> MNSLSSKKANSLVFKSIRNFTLQWGSLAERPMVDRVMSTSTWPVPYYQRLFKAYPIREKKDKMSLLLSDIDIDDTNWYQAKDFLRGSFRGRQIVDYVENNIASNTYILI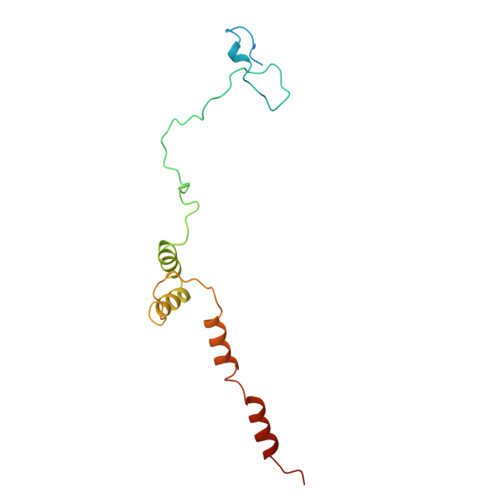QQDVANMAKAYVHDICGYIDVANKENVRILSKGDLI(S,S)-(-)-N,N'-DI-5'-[5',6',7',8'-TETRAHYDRO- 2'(1'H)-QUINOLYNYL]-1,12-DIAMINODODECANE DIHYDROCHLORIDE | C30 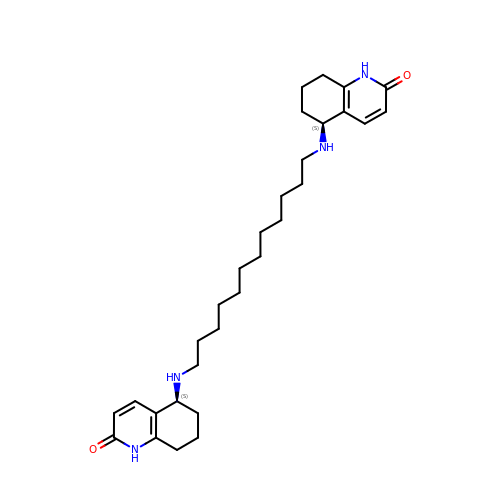H46 N4 O2 | VFFGYPZORQBRNM-UIOOFZCWSA-N>GSTLVTGSEYETMLTEIMSMGYERERVVAAL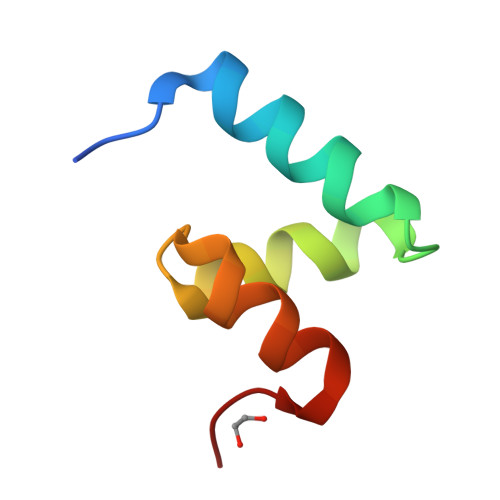RASGNNPHRAVEYLLTGIPG[2x]> ADSRIRIRGYVR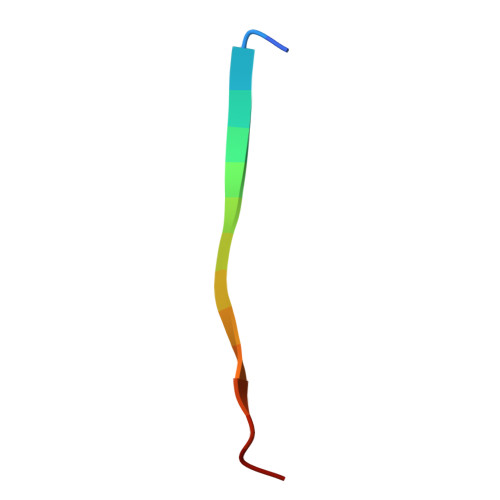NNG>[2x]MMFNFYQFLYNLQNVSPFIDFSVLKQLTHTKMRENEPARFETRSFSQLIDHARSWKTEVRGMTTQGFTKISLMRAEKDRLNMYAISSVPGTNTQSIFSVTIPLELVEKAQVADRKFELKLKSGYNVDSYIRKTPPSAEFTLQCERQRSQVVTGISDYEIRNGKMILMAGDQLFRYNPLNEALAAIPIAVPDDQSSTEPMDISEGSITSGTKGSGSEAPQSSTVPPVTRIPIKKPTTSTEKPATAPPTNNFVSSAKVCP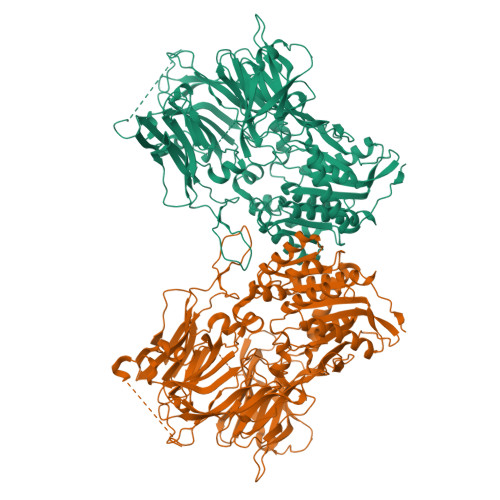ADSSLLAYVLNKQVYIEKNGKIIHRTSSNSKHITNGVPSYIVQEELERFEGIWWSESKTRLLYEHVNEEKVAESQFGVNGDPPVAPMKYPRAGTKNAYSTLRMVILENGKAYDVPLKDEVIYKHCPFYEYITRAGFFSDGTTVWVQVMSRDQAQCSLLLIPYTDFLLPEELGGSIKEDNLQLSTDLNMGVWDDKSHEETMEKPPRGKLRGTVQIHKARNDYWINTHNAIYPLKITDEEHPMYEFIYCLEKPNGSCLALISAELDQNGYCRHTEEKLLMAENFSINKSMGIVVDEVRELVYYVANESHPTEWNICVSHYRTGQHAQLTESGICFKSERANGKLALDLDHGFACYMTSVGSPAECRFYSFRWKENEVLPSTVYAANITVSGHPGQPDLHFDSPEMIEFQSKKTGLMHYAMILRPSNFDPYKKYPVFHYVYGGPGIQIVHNDFSWIQYIRFCRLGYVVVFIDNRGSAHRGIEFERHIHKKMGTVEVEDQVEGLQMLAERTGGFMDMSRVVVHGWSYGGYMALQMIAKHPNIYRAAIAGGAVSDWRLYDTAYTERYMGYPLEEHVYGASSITGLVEKLPDEPNRLMLVHGLMDENVHFAHLTHLVDECIKKGKWHELVIFPNERHGVRNNDASIYLDARMMYFAQQAIQGFGPTTAAPRQGPLWSHPQFEK>[5x]MDFSRNLYDIGEQLDSEDLASLKFLSLDYIPQRKQEPIKDALMLFQRLQEKRMLEESNLSFLKELLFRINRLDLLITYLNTRKEEMERELQTPGRAQISAYRVMLYQISEEVSRSELRSFKGGLQEEISKCKLDDDMNLLDIFIEMEKRVILGEGKLDILKRVCAQINKSLLKIINDYEEFSKER;>[4x]MSAEVIGQVEEALDTDEKEMLLFLCRDVAIDVVPPNVRDLLDILRERGKLSVGDLAELLYRVRRFDLLKRILKMDRKAVETHLLRNPHLVSDYRVLMAEIGEDLDKSDVSSLIFLMKDYMGRGKISKEKSFLDLVVELEKLNLVAPDQLDLLEKCLKNIHRIDLKTKIQKYKQSVQGAGTS;> MDPFLVLLGSVSSSLSSSELTELKFLCLGRVGKRKLERVQSGLDLFSMLLEQNDLEPGHTELLRELLASLRRH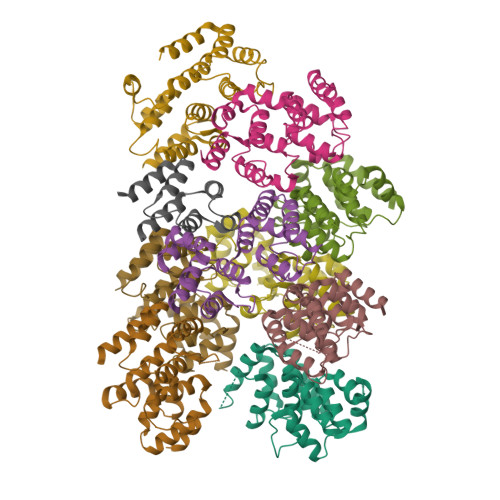DLLRRVDDFEAGAAAGAAPGEEDLCAAFNVICDNVGKDWRRLARQLKVSDTKIDSIEDRYPRNLTERVRESLRIWKNTEKENATVAHLVGALRSCQMNLVADLVQEVQQARDLQNRSGAMSPMSWNSDASTSEASLEHHHHHH> MSELEKAVVALIDV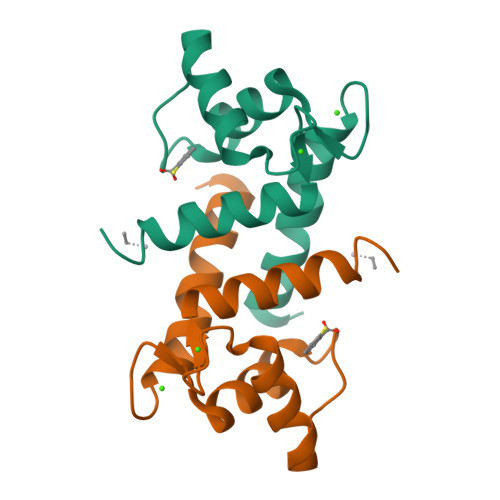FHQYSGREGDKHKLKKSELKELINNELSHFLEEIKEQEVVDKVMETLDSDGDGECDFQEFMAFVAMITTACHEFFE We studied one type III effector from plant pathogenic bacteria called Pseudomonas syringae. This effector, termed avirulence protein B (AvrB), is targeted to the inner face of the plant cell plasma membrane, where it interacts with a membrane-bound host protein called RIN4 (resistance to Pseudomonas maculicula protein–interacting protein). A crystal structure of free AvrB revealed that it adopts a novel bilobal fold with no structural homologies to previously characterized proteins or functional domains. The junction of the two lobes forms a large solvent-accessible cleft with a volume of over 900 Å3 that extends into the lower lobe to form a pocket rich in conserved residues. Our data significantly extend previous observations defining the key functional regions of the type III effector protein AvrB: its upper lobe and interlobal cleft mediate contact with the Arabidopsis target protein RIN4, and the lower lobe contains a pocket suitable for binding ADP or another similarly shaped molecule.

The structure of AvrB complexed to RIN4142–176 revealed that the peptide forms a “Z” shape with the N-terminal half contacting the upper lobe and the C-terminal half straddling the interface between the two lobes. The interaction of AvrB with RIN4142–176 does not alter the overall structure of AvrB (unpublished data). The N-terminal half of RIN4142–176 interacts mainly through hydrophobic burial of RIN4 W154 plus a hydrogen bond between the indole nitrogen of RIN4 W154 and AvrB D213. The most extensive interactions of RIN4142–176 with AvrB involve the C-terminal half of the RIN4 peptide. First, there is a set of antiparallel beta-strand hydrogen-bonding interactions between main-chain AvrB residues 120 to 124 (within strand β1) and RIN4 residues 167–171. Second, there is a hydrogen bond between the main-chain of RIN4 N170 and the AvrB R209 guanidinium group. These interactions allow this region of RIN4 to form an additional strand of the beta-sheet in the upper lobe of AvrB. Importantly, in forming this strand, the RIN4 T166 side-chain is directed toward the interior of AvrB such that the hydroxyl group hydrogen bonds with the hydroxyl group of AvrB T125, which in turn hydrogen bonds to the imidazole ring of AvrB H217. Above this hydrogen-bonding arrangement, the aromatic rings of RIN4 Y165 and F169 as well as interleaving H167 are thrust against the surface formed from the last two turns of AvrB helix α7. The guanidinium groups of AvrB R209 and AvrB R266 buttress the termini of the ring-stack, contacting RIN4 F169 and Y165, respectively, via π–π interactions such that the guanidium groups are also almost parallel to the three stacked aromatic rings of RIN4.

>[2x]GAMGCVSSKSTTVLSPQTSFNEASRTSFRALPGPSQRQLEVYDQCLIGAARWPDDSSKSNTPENRAYCQSMYNSIRSAGDEISRGGITSFEELWGRATEWRLSKLQRGEPLYSAFASERTSDTDAVTPLVKPYKSVLARVVDHEDAHDEIMQDNLFGDLNVKVYRQTAYLHGNVIPLNTFRVATDTEYLRDRVAHLRTELGAKALKQHLQRYNPDRIDHTNASYLPIIKDHLNDLYRQAISSDLSQAELISLIARTHWWAASAMPDQRGSAAKAEFAARAIASAHGIELPPFRNGNVSDIEAMLSGEEEFVEKYRSLLDSDCF;>[2x]PEKVTVVPKFGDWDENNPSSADGYTHIFNKVREER>MRSSKIRCPGAIRVGTLVTAFGCLPHVAFAAAREAPPVTPEVLVRLADIGTMSASETTPLLSLSPDGRYVAFQVRQADPVTNLNVFRMVVKATDGATDAIDVDVGGEYLFWTIPSWGYARNAPSGANLTIQPRWSPSGTHLAYLRQDQGRVRVWRASVKGEGASPVIEDAYDIEDVQWLDDNTLIYSGRPGFVEAEAEIEREGRRGWVYDERFHPLTGARPRVLEPISIVYQVLDLKTGTRRAATPTEVARLREKPDPLRAMVGRTTFSVSRTDPQNINAPTTLVARRGEGEPVRCDEEACQNITRMWGDETANVLYFLRREGWASNEMALYRMPADALKPVRIWHATGLLQGCERQAKRLICAQESALQPRRLVTLNLTSGQMSPLYDPNPDLSRYRLPKVERLTLRNRNGIEVFSDLVLPPDYQLGTRLPLVIVQYSSRGFLRGGTGDENPILPLATAGFAVLSFHSPRSEASYQRFTSPIA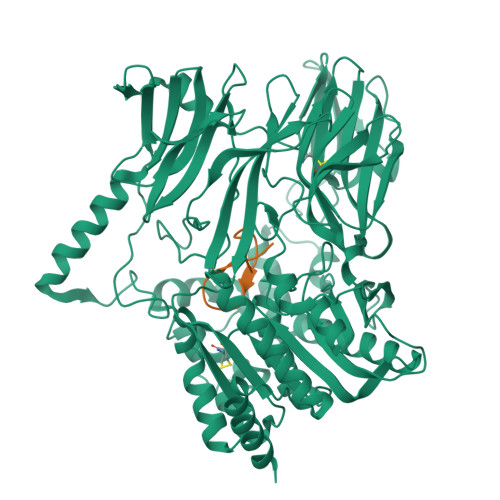QSKAEYSNWRNRWNILHTLEDLIDDLDRRGVIDPARVGLTGLADGATTVHFGLINSHRFAAAVTSSCCTDSFTASVMNGPRISGALKAYGIETDQADDGPFWAATSFVVNASRLDTPLLIQSADEEYLGALPGFTALQQARKPVELIIYPNEHHVKWQPAHRLAVYNRTIDWFRFWLMDQSDPAPDKAAQYDRWRALRALRQKSPSPTPAPGSRSHHHHHH[2x];>[2x]GPTPMVGLDSVSGQYWDQHAPLAD> GSSHHHHHHSSGRENLYFQGHMLQFYRNLGKSGLRVSCLGLGTWVTFGGQITDEMAEQLMTLAYDNGINLFDTAEVYAAGKAEVVLGNIIKKKGWRRSSLVITTKIFWGGKAETERGLSRKHIIEGLKASLERLQLEYV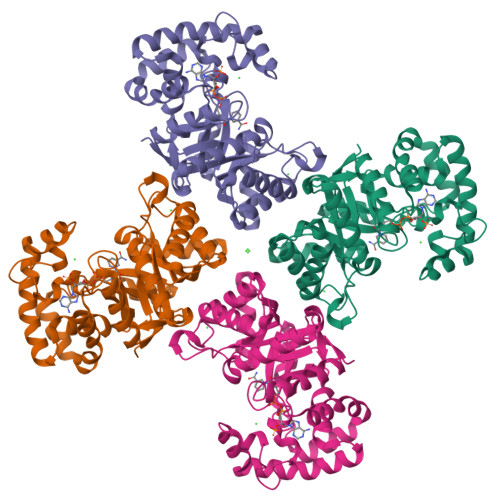DVVFANRPDPNTPMEETVRAMTHVINQGMAMYWGTSRWSSMEIMEAYSVARQFNLTPPICEQAEYHMFQREKVEVQLPELFHKIGVGAMTWSPLACGIVSGKYDSGIPPYSRASLKGYQWLKDKILSEEGRRQQAKLKELQAIAERLGCTLPQLAIAWCLRNEGVSSVLLGASNADQLMENIGAIQVLPKLSSSIIHEIDSILGNKPY> EEYSSNWAGAVLIGDGYTKVTGEFTVPSVSAGSSGSSGY;> QSEEYCASAWVGIDGDTCETAILQTGVDFCYEDGQTSYDAWYEWYPDYAYDFSDITISEGDSIKVTVEATSKSSGSATVENLTTGQSVTHTFSGNVEGDLCETNAEWIVEDFESGDSLVAFADFGSVTFTNAEATSGGSTVGPSDATVMDIEQDGSVLTETSVSGDSVT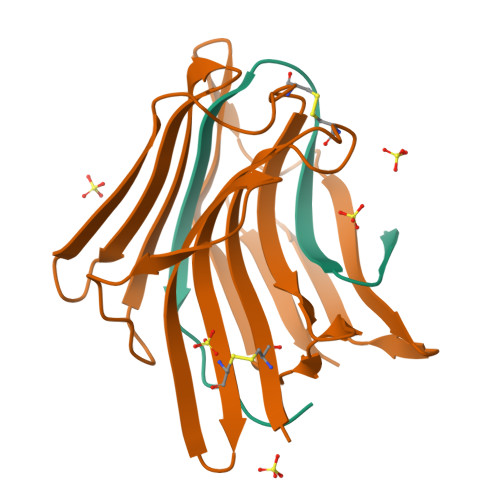VTYV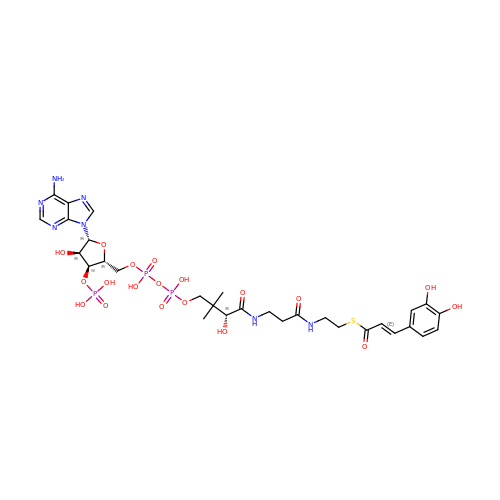S-[2-[3-[[(2R)-4-[[[(2R,3S,4R,5R)-5-(6-aminopurin-9-yl)-4-oxidanyl-3-phosphonooxy-oxolan-2-yl]methoxy-oxidanyl-phosphoryl]oxy-oxidanyl-phosphoryl]oxy-3,3-dimethyl-2-oxidanyl-butanoyl]amino]propanoylamino]ethyl] (E)-3-[3,4-bis(oxidanyl)phenyl]prop-2-enethioate | C30 H42 N7 O19 P3 S | QHRGJMIMHCLHRG-ZSELIEHESA-N6-~{tert}-butyl-8-fluoranyl-2-[3-(hydroxymethyl)-4-[1-methyl-5-[[5-(1-methylpiperidin-4-yl)pyridin-2-yl]amino]-6-oxidanylidene-pyridazin-3-yl]pyridin-2-yl]phthalazin-1-one | C34 H37 F N8 O3 | 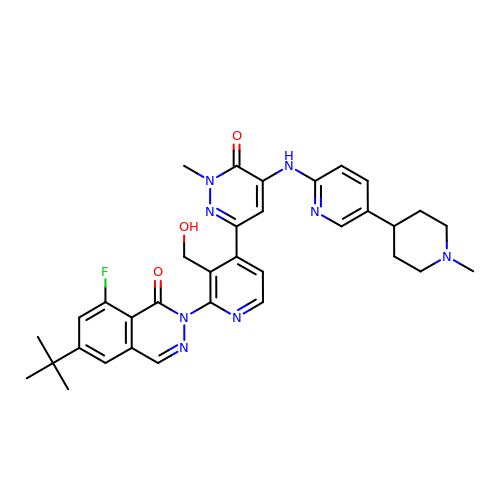YPYHTXOIYCWSMJ-UHFFFAOYSA-N The Luteoviridae are an important family of pathogenic viruses responsible for necrosis of the plant vasculature which, in turn, causes severe stunting and dwarfism, and ultimately crop loss. The structures for BYDV and PLRV each reveal a luteovirid capsid composed of 180 CP monomers. The CP monomers each contain a single canonical jellyroll fold, and are arranged with T = 3 icosahedral quasi-symmetry to give a particle with a diameter of ∼30 nm. The luteovirid capsids are formed from CP subunits with a canonical jellyroll fold comprising two opposing β sheets, each containing 4 antiparallel β strands (βB-βI).

We therefore present high-resolution structures for VLPs of BYDV and PLRV at 3.0-Å and 3.4-Å resolution, respectively. BYDV and PLRV CPs assembled into monodisperse, homogeneous particles of the anticipated diameter. When imaged in ice, both BYDV and PLRV VLPs were monodisperse, so cryo-EM datasets were collected for each (see STAR Methods). Structure refinement was carried out with icosahedral symmetry imposed, yielding density maps at a resolution of 3.0 Å for BYDV and 3.4 Å for PLRV (see Table S1 for refinement statistics). Density maps for each structure were of sufficient quality and resolution to allow for unambiguous building of the shell (S) domain of the CP (BYDV: residues 61–200∗; PLRV: residues 68–208). In both cases the N-terminal R (RNA-binding) domain is not resolved in the cryo-EM density, except in the “C” conformer of BYDV, where an additional six residues of the R domain (residues 55–60) are visible. No density for such metal ions is seen in either BYDV or PLRV, and no putative metal binding sites were identified using bioinformatics. As for many viruses, both capsid structures are strongly positively charged on their inner surfaces, presumably to help facilitate packaging of the polyanionic RNA genome. The outer surface charge profile is similar in both BYDV and PLRV capsid structures, with an acidic patch at the center of each asymmetric trimer. Inspection of the interfaces between individual CP protomers, and between asymmetric units, in BYDV and PLRV suggest that both viruses have a similar volume of solvent hidden surface involved in supramolecular assembly. BYDV and PLRV have comparatively short insertions at the C-D, E-F, and G-H loops, where larger insertions are found in all other viruses with known structures, resulting in a much more compact fold.

>[3x]MNSVGRRGPRRANQNGTRRRRRRTVRPVVVVQPNRAGPRRRNGRRKGRGGANFVFRPTGGTEVFVFSVDNLKANSSGAIKFGPSLSQCPALSDGILKSYHRYKITSIRVEFKSHASANTAGAIFIELDTACKQSALGSYINSFTISKTASKTFRSEAINGKEFQESTIDQFWMLYKANGTTTDTAGQFIITMSVSLMTAK>[3x]MGAMIVKEVYETAEKIKSMEIRGAGRIARAAAQALMIQAEKSKAKEPEELWNELKVASKILYNTRPTAVSLPNALRYVMHRVKAAYLGGADLET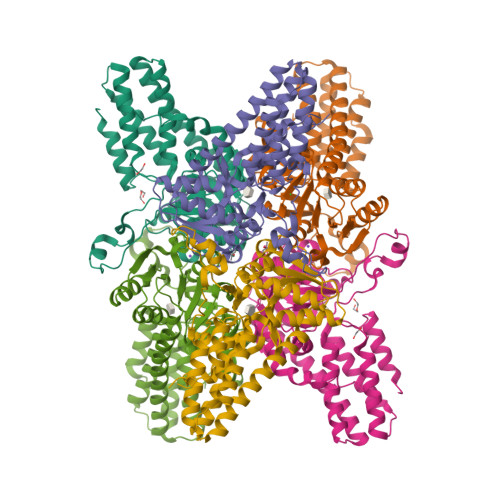LRFTAINSAKEFIYNSEKAIERIGEIGAKRIEDGDIIMTHCHSKAAISVMKKAFEQGKNIKVIVTETRPKWQGKITAKELASYGIPVIYIVDSAARHYMKMTDKVVMGANSITANGAVINKIGTSLIALTAKEHRVWVMIAAETYKFHPATMLGQLVEIEMRDPTEVIPEEELRTWPKNIEVWNPAFDVTPPEYIDVIITERGIIPPYAAIDILKEEFGWALKYKEPWED> RIAISNSNRTRSVPSLTTIWSISPTPNCSIYETQDANLFLCLTKNGAHVLGTITIKGLKGALREMHDNALSLKLPFDNQGNLLNCALESSTWRYQETNAVASNALTFMPNSTVYPRNKTAHPGNMLIQISPNITFSVVYNEINSGYAFTFKWSAEPGKPFHPPTAVFCYITEQGSHH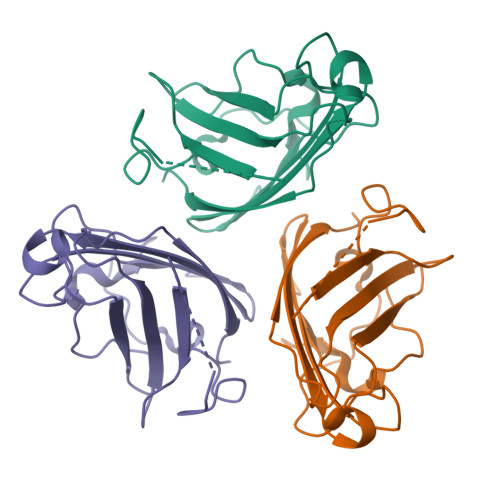HHHH~{N}-[3-(3,5-dimethyl-1,2-oxazol-4-yl)-5-(5-ethanoyl-2-ethoxy-phenyl)phenyl]furan-2-carboxamide | C26 H24 N2 O5 | 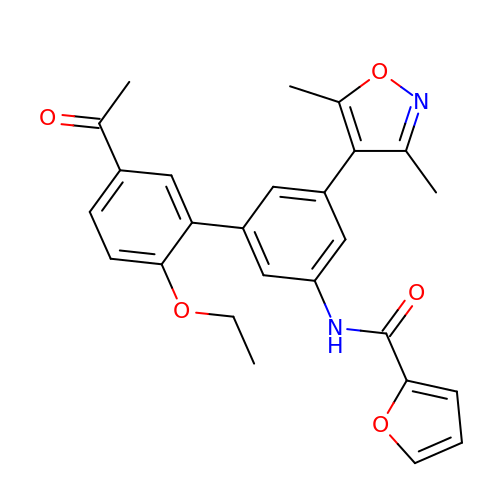WQLADCZJBORKGE-UHFFFAOYSA-N> MVDDAGAAESQRGKQTPAHSLEQLRRLPLPPPQIRIRPWWFPVQELRDPLV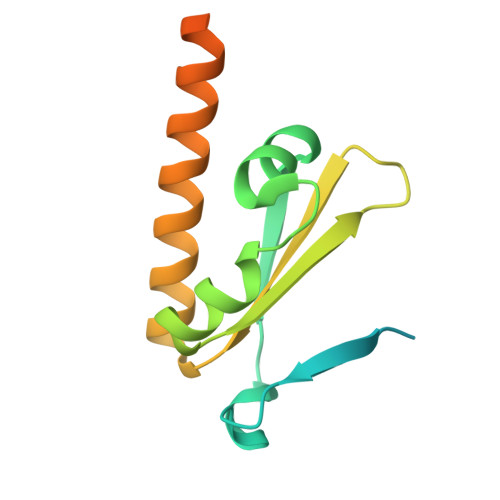FYLEAWLADELFGPDRAIIPEMEWTSQALLTVDIVDSGNLVEITVFGRPRVQNRVKSMLLCLAWFHREHRARAEKMKHLEKNLKAHASDPHSPQDPVA> GAHMSYSYDAPSDFINFSSKQKNEESKKRQWALEDFEIGRPLGKGKFGNVYLAREKQSKFILALKVLFKAQLEKAGVEHQLRREVEIQSHLRHPNILRLYGYFHDATRVYLILEYAPLGTVYRELQKLSKFDEQRTATYITELANALSYCHSKRV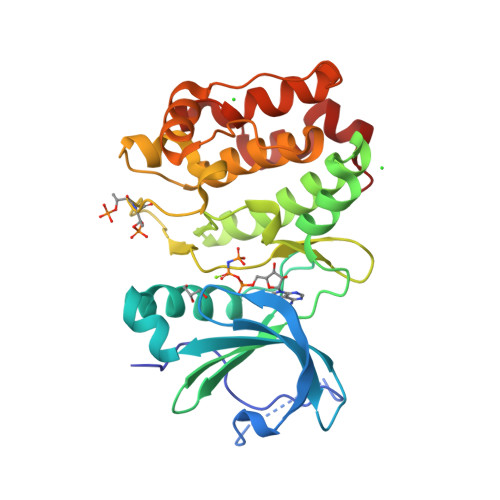IHRDIKPENLLLGSAGELKIADFGWSVHAPSSRRTTLCGTLDYLPPEMIEGRMHDEKVDLWSLGVLCYEFLVGKPPFEANTYQETYKRISRVEFTFPDFVTEGARDLISRLLKHNPSQRPMLREVLEHPWITANSSK>MAEKTFKVVSDSGIHARPATILVQTASKWNSEIQLEYNGKTVNLKSIMGVMSLGIPKGATIKITAEGADAAEAMAALTDTL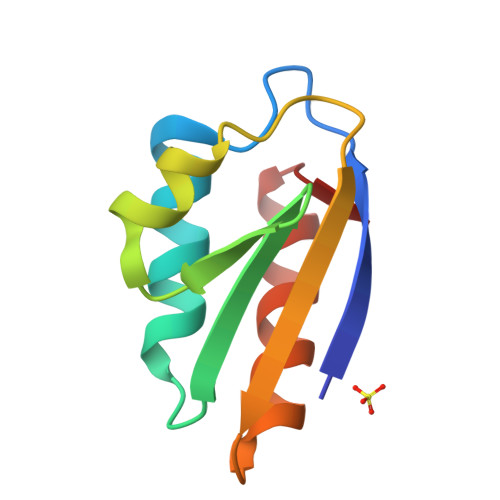AKEGLAE[3x]>TDENQTIQNDSSSSLTQVNTTMSVQMDKKALLCCFSSPLINAVLITWIIKHRHLPSCTIAYNLDKKTNETSCLGRNITWASTPDHSPELQISAVALQHEGTYTCEIVTPEGNLEKVYDLQVLVPPEVTYFPGKNRTAVCEAMAGKPAAQISWT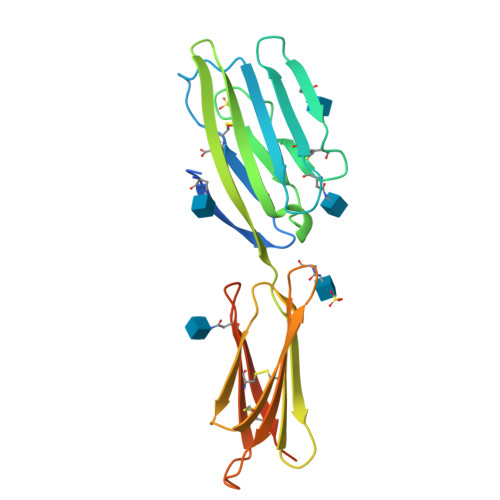PDGDCVTKSESHSNGTVTVRSTCHWEQNNVSVVSCLVSHSTGNQSLSIELSQGTMTTPRSTRHHHHHH[3x]>[18x]MGHNNTKGNRKFIKGRYTANAAKGE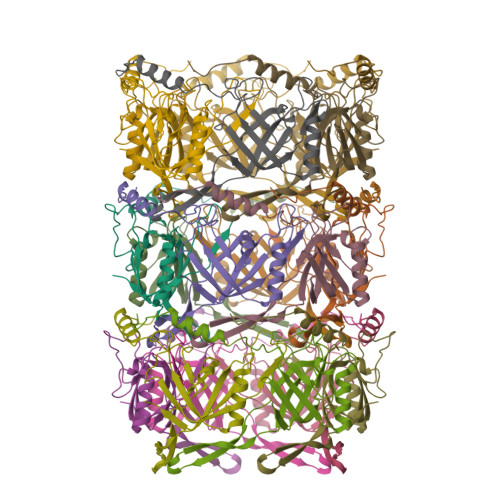RLVSSEFLLTFAGHEDISVLVRTSQIPEMTREDVEDYGPNGVKFNQHGPIRNSGEIQVQCVETIEGDILQFIKDRIAAKDYVDITMAATPESKSSGVNAVTKAATTIEMLDCKIYSDAIDFSTEDVTAAVRPSLRIVYNWIEWD> GRKTEKVVNNGIPWFDDRGEIVNAHGACIVEENGRYYLFGEYKSDKSNAFPGFSCYSSDDLVNWKFERVVLPMQSSGILGPDRVGERVKVMKCPSTGEYVMYMHADDMNYKDPHIGYATCSTIAGEYKLHGPLLYEGKPIRRWDMGTYQDTDGTGYLLLHGGIVYRLSKDYRTAEEKVVSGVGGSHGESPAMFKKDGTYFFLFSNLTSWEKNDNFYFTAPSVKGPWTRQGLFAPEGSLTYNSQTTFVFPLKCGEDTIPMFMGDRWSYPHQASAATYVWMPMQVDGTKLSIPEYWPSWDVDKLKPVNPLRKGKTVDLKKITFSKEADWKVEEGRISSNVKGSTLSIPFTGSCVAVMGETNCHSGYARMNILDKKGEKIYSSLVDFYSKANDHATRFKTPQLAEG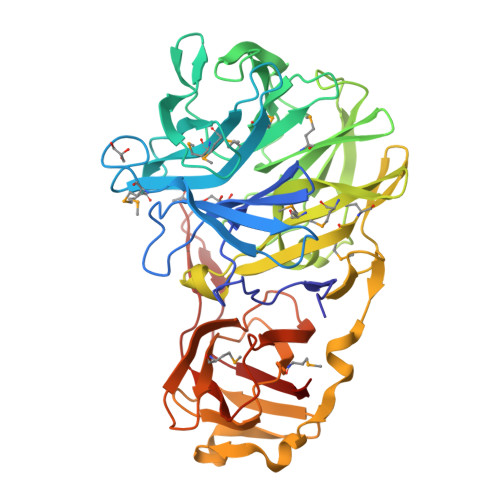EYTLVIEVTGISPTWTDKTKRIYGSDDCFVTITDIVKL>[2x]MNPTIIRARAPLRLGLAGGGTDVAPYADTFGGYVLNATIDRYAYAVIKTLTIPAVRFVSTDQQVEKHQLISEPLELNGTLNLHKAVYNHMIRNYNHGKPIALELSTFCDAPAGSGLGSSSTLVVVMIKAFVELLNLPLDDYAIAQLAYRIERVDCGLAGGRQDQYSATFGGFNFMEFYAAARTIVNPLRIKNWVLCELEASLVLFYTGVSRESAKIIQDQSDNVVSHKTAAIEAMHGIKREALVMKEALLKGDFKAFVASMRLGWDNKKNSARTVSNAHIDEIYDAAIRAGAQAGKVSGAGGGGFMLFFVPTEKRMDLIRTLGEYDGQVSNCHFTKNGTQAWRIAN

Here, we present the structure of WcbL from Burkholderia pseudomallei. A critical step in the synthesis of heptoses is their 1-O phosphorylation, mediated by kinases such as HldE or WcbL. We report that WcbL operates through a sequential ordered Bi-Bi mechanism, loading the heptose first and then ATP. The protein forms a head-to-tail dimer, with the two active sites facing away from the dimer interface, in line with the native molecular weight predicted from size-exclusion chromatography.

To improve our understanding of WcbL, we solved the crystal structure of the enzyme to 1.78 Å resolution. The structure was solved using the single-wavelength anomalous dispersion (SAD) method, using selenomethionine-labeled protein to provide a strong anomalous signal. The solved structure reveals that WcbL adopts, as expected, the GHMP sugar kinase fold. Native crystals formed in a number of related space groups in identical conditions, and determining the correct space group was challenging for many crystals. Native WcbL and an AMP-PNP complex had a lower proportion of the monoclinic fraction: for these complexes data did not process well and the model did not refine in the monoclinic space group. Comparison of the sequence with galactokinases reveals a Q-L mutation at position 162. This facilitates the accommodation of the extra carbon unit in the heptose sugar compared with the hexose substrate of the related enzymes. The native state shows a structure with strong stability: most of the structural elements are built from hydrogen bonds of 4.1 kcal/mol or greater.> MINGVYYNEISRDLDISSSTQCLRFLKETVIPSLANNGNNSTSIQYHGISKNDNIKKSVNKLDKQINMADRSLGLQQVVCIFSYGPHIQKMLS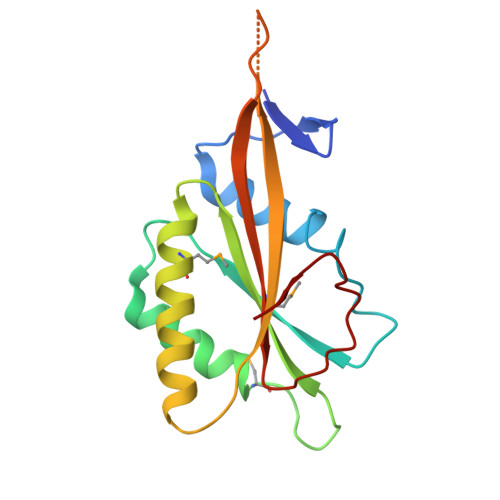ILEIFKKGYIKNNKKIYQWNKLTSFDIKREGRNELQEERLKVPILVTMVSDSEIIDLNLHSFTKQ>MGKYQVMKRASEVDLSTVKYKAETMKAPHLTGLSFKLFVNLLEAPLIGSLIVDYLKKDNGMTKIFRNTVIPEEPMFRPEFPSQEPEHDVVIVGEDESPIDRLETALKCLPQYDPSRSLHADPVSSFRYWKIRDYAYAYRSKLTTPLQVAKRIISIIEEFGYDKPPTPFLIRFDANEVIKQAEASTRRFEQGNPISVLDGIFVTIKDDIDCLPHPTNGGTTWLHEDRSVEKDSAVVSKLRSCGAILLGKANMHELGMGTTGNNSNYGTTRNPHDPKRYTGGSSSGSAAIVAAGLCSAALGTDGGGAVRIPSALCGITGLKTTYGRTDMTGSLCEGGTVEIIGPLASSLEDAFLVYAAILGSSSADRYNLKPSPPCFPKLLSHNGSNAIGSLRLGKYTKWFNDVSSSDISDKCEDILKLLSNNHGCKVVEIVVPELEEMRAAHVISIGSPTLSSLTPYCEAGKNSKLSYDTRTSFAIFRSFSASDYIAAQCLRRRLMEYHLNIFKDVDVIVTPTTGMTAPVIPPDALKNGETNIQVTTDLMRFVLAANLLGFPAISVPVGYDKEGLPIGLQIMGRPWAEATVLGLAAAVEELAPVTKKPAIFYDILN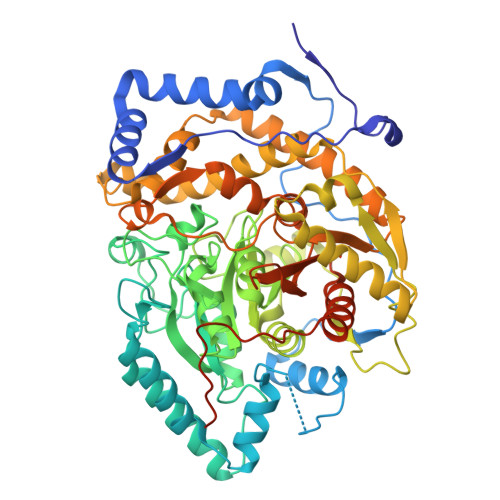TNKGEFEAYVEQKLISEEDLNSAVDHHHHHH[2x]> GQDRSEATLIKRFKGEGVRYKAK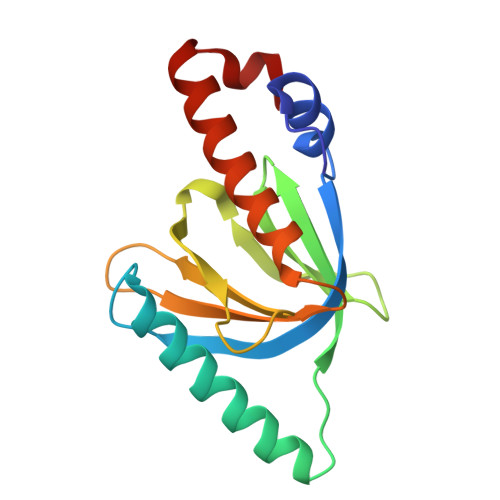LIGIDEVSAARGDKLCQDSMMKLKGVVAGARSKGEHKQKIFLTISFGGIKIFDEKTGALQHHHAVHEISYIAKDITDHRAFGYVCGKEGNHRFVAIKTAQAAEPVILDLRDLFQLIYELKQREELEKKA> LPLRESHTAHQATDFGVKVFQQVVQASKD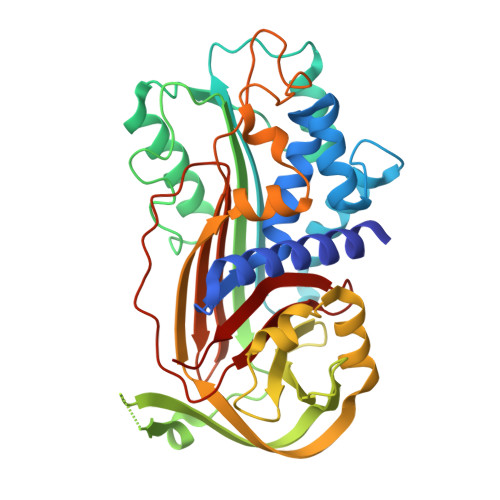RNVVFSPYGVSSVLAMLQMTTAGKTRRQIQDAMGFKVNEKGTAHALRQLSKELMGPWNKNEISTADAIFVQRDLELVQGFMPHFFKLFQTMVKQVDFSEVERARFIINDWVERHTKGMINDLLAKGAVDELTRLVLVNALYFSGQWKTPFLEASTHQRLFHKSDGSTVSVPMMAQSNKFNYTEFTTPDGLEYDVVELPYQGDTLSMFIAAPFEKDVHLSALTNILDAELIRQWKGNMTRLPRLLILPKFSLETEVDLRGPLEKLGMPDMFSATLADFTSLSDQEQLSVAQALQKVRIEVNESGTVASSSTAFVISARMAPTEMVIDRSFLFVVRHNPTETILFMGQVMEP>[2x]ATAVNGAPRDAALWSSHEQMLAQPLKDSDAEVYDIIKKESNRQRVGLELIASENFASRAVLE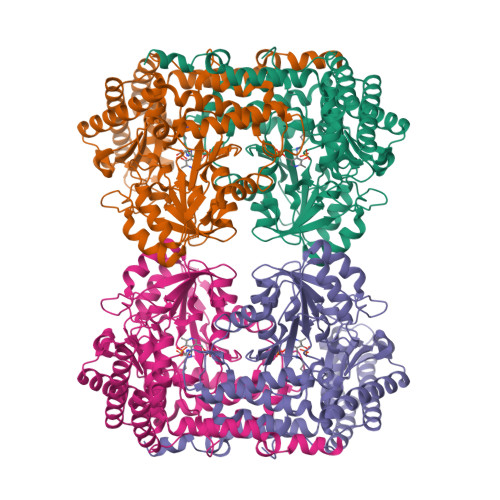ALGSCLNNKYSLGYPGQRYYGGTEHIDELETLCQKRALQAYGLDPQCWGVNVQPYSGSPANFAVYTALVEPHGRIMGLDLPDGGHLTHGFMTDKKKISATSIFFESMAYKVNPDTGYIDYDRLEENARLFHPKLIIAGTSCYSRNLDYGRLRKIADENGAYLMADMAHISGLVVAGVVPSPFEHCHVVTTTTHKTLRGCRAGMIFYRRGVRSVDPKTGKEILYNLESLINSAVFPGLQGGPHNHAIAGVAVALKQAMTPEFKEYQRQVVANCRALSAALVELGYKIVTGGSDNHLILVDLRSKGTDGGRAEKVLEACSIACNKNTCPGDKSALRPSGLRLGTPALTSRGLLEKDFQKVAHFIHRGIELTVQIQDDTGPRATLKEFKEKLAGDEKHQRAVRALRQEVESFAALFPLPGLPGF> GSGAG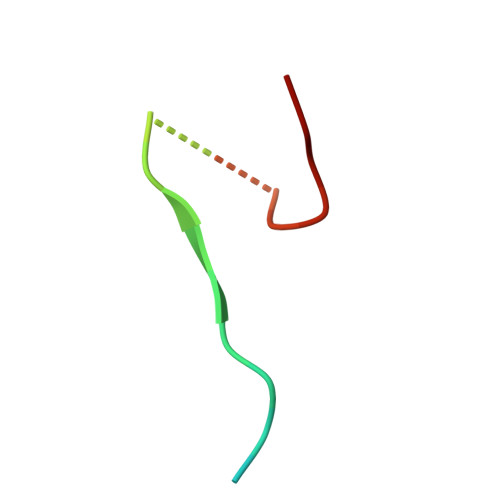EAEERVVVISSSEDSDAENSSSRY> MNINQLILRNLKKNLRNYYLYVFALIFSVALYFAFVTLQYDPAINEVKASIKGAAAIKTASILLVAVVAIFILYANTIFIKRRSKEIGLFQLIGMTKHKIFRILSAENVMLYFGSLAIGVAAGFSISKLVLMILFKIVDVKADAKLHFSEQALVQTVIVFCGIYLLIMIMNYTFIKKQSILSLFKVTSSTEDKVKKISFFQMLIGALGIVLILTGYYVSSELFGGKFKTINELFVAMSFILGSVIIGTFLFYKGSVTFISNIIRKSKGGYLNISEVLSLSSIMFRMKSNALLLTIITTVSALAIGLLSLAYISYYSSEKTAEQNVAADFSFMNEKDAKLFENKLRESNISFVKKATPVLQANVDIANIMDGTPKEMQGDPGNMQLAVVSDKDVKGVDVAAGEAVFSGYTDLLQKIMVFKDSGVIKVKSKHETQPLKYKGLREEFLVSYTFTSGGMP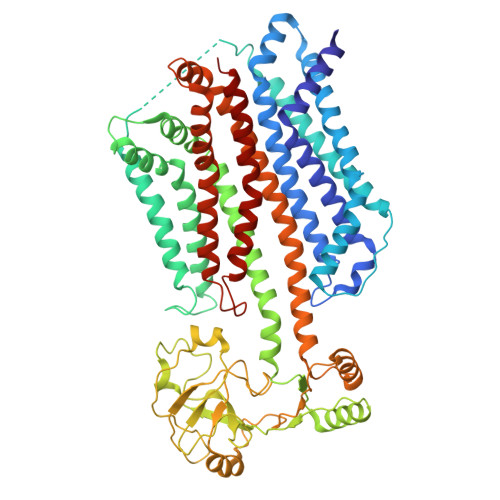AVIVDDSLFKQLDKDKDPRIQLAQSTFIGVNVKHDDQMEKANELFQQVNKKNEHLSRLDTSAAQKSLFGMVMFIVGFLGLTFLITSGCILYFKQMGESEDEKPSYTILRKLGFTQGDLIKGIRIKQMYNFGIPLVVGLFHSYFAVQSGWFLFGSEVWAPMIMVMVLYTALYSIFGFLSVLYYKKVIKSSL> APGDLLWSDEFDGAAGSAPNPAVWNHETGAHGWGNAELQNYTASRAN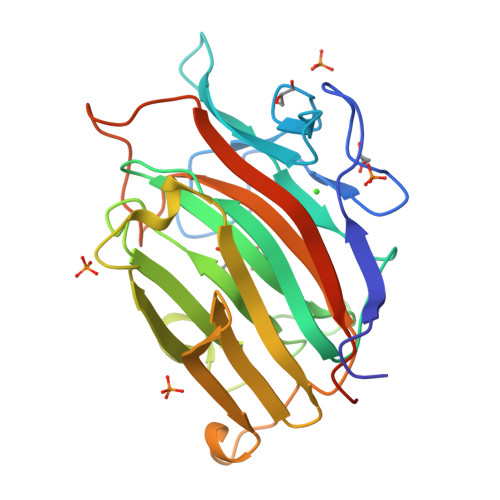SALDGQGNLVITARREGDGSYTSARMTTQGKYQPQYGRIEARIQIPRGQGIWPAFWMLGGSFPGTPWPSSGEIDIMENVGFEPHRVHGTVHGPGYSGGSGITGMYQHPQGWSFADTFHTFAVDWKPGEITWFVDGQQFHRVTRASVGANAWVFDQPFFLILNVAVGGQWPGYPDGTTQLPQQMKVDYVRVYDNGSGSSNPGNPGTGLPT>[6x]MYKHTIVYDGEVDKI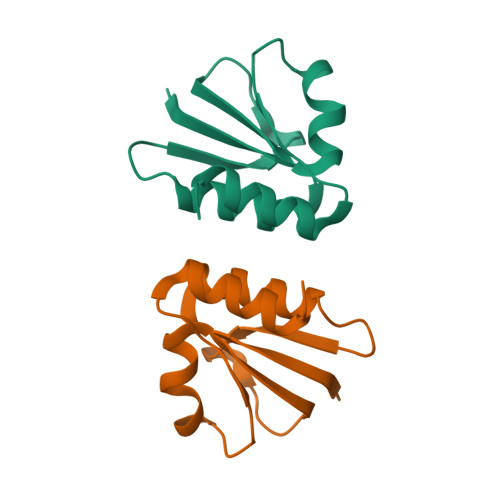SATVVGWGYNDGKILICDIKDYVPGQTQNLYVVGGGACEKISSITKEKFIMIKGNDRFDTLYKALDFINR> GMDVTIERVNDFDGYNWLPLLAKSSQEGFQLVERMLRNRREESFQEDGEAMFVALSTTNQVLACGGYMKQSGQARTGRIRHVYVLPEARSHGIGTALLEKIMSEAFLTYDRLVLYSEQADPFYQGLGFQ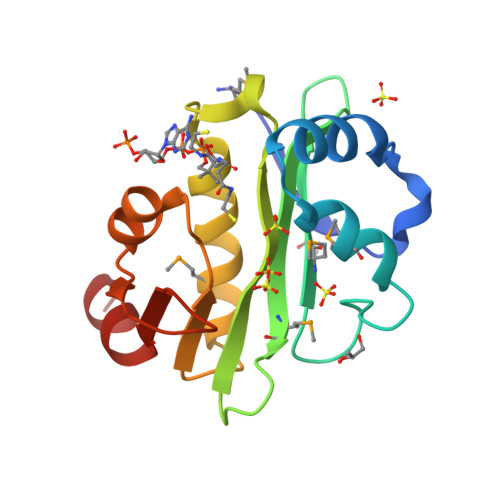LVSGEKITHTLDKTAFADSNR>GSHMDFEIEVMNYSIEEFREFKTTDVESVLPFRDSSTPTWINITGIHRTDVVQRVGEFFGIHPLVLEDILNVHQRPKVEFFENYVFIVLKMFTYDKNLHELESEQVSLILTKNCVLMFQEKIGDVFDPVRERIRYNRGIIRKKRADYLLYSLIDALVDDYFVLLEKI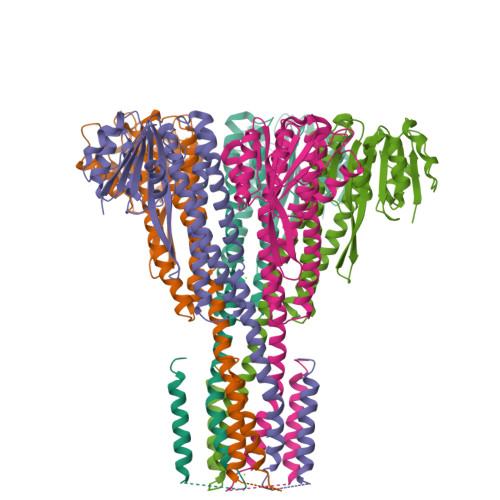DDEIDVLEEEVLERPEKETVQRTHQLKRNLVELAATIWPLREVLSSLYRDVPPLIEKETVPYFRDVYDHTIQIADTVETFRDIVSGLLDVYLSSVSNKTNEVMKVLTIIATIFMPLTFIAGIYGMNFEYMPELRWKWGYPVVLAVMGVIAVIMVVYFKKKKWL[5x]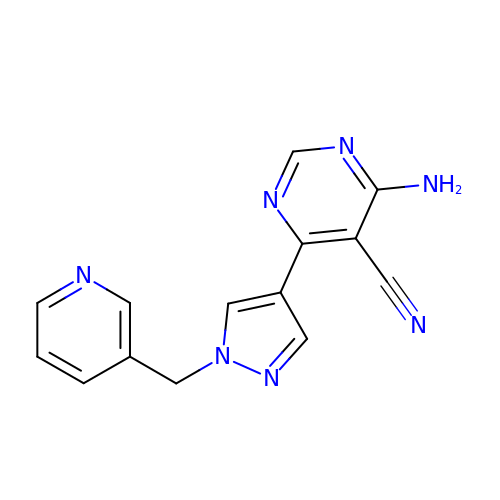4-azanyl-6-[1-(pyridin-3-ylmethyl)pyrazol-4-yl]pyrimidine-5-carbonitrile | C14 H11 N7 | CXHWYZDXLJBAJA-UHFFFAOYSA-N> MSGMPPRVRRRVEELLR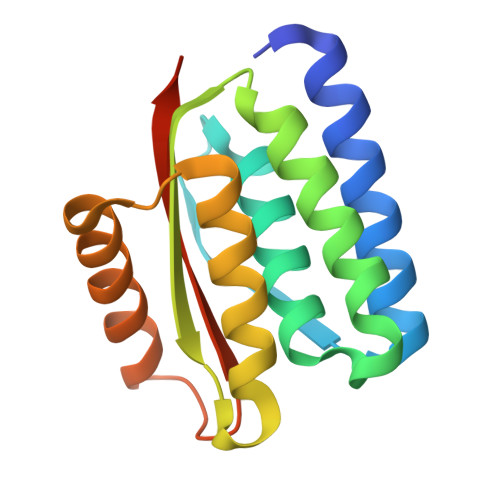RARELAEELGIRVEVLEVDPEYELELTAVITLAILAVLAPPERQDEVLELLRETLKTLSEVVESLAVSIWAPPEREEAARRVERLVEEAFNTTPETRERARKLRDEARRDAEPDEVVVAVHLVPKGSHHHHHH Here, we describe and detail the use of sub-particle CryoEM averaging and present updated reconstructions of DARP14, a multi-subunit tetrahedrally symmetric protein complex. Originally described by Liu and Gonen et al. (2018), DARP14 was computationally designed as a scaffold capable of displaying small proteins for CryoEM. DARPins are small, ~17 kDa helical repeat proteins that feature variable residue loops capable of selective non-covalent binding to other proteins, akin to antibodies. Variants of DARP14 and similar scaffolds have since been generated and used to bind and image small proteins, such as GFP and KRAS.

In addition to focusing on the DARPin components, we also set out to extract as much high-resolution information as possible from the stable core cage component, this time by masking out the dynamic parts of the complex. To push for the highest resolution possible given the dataset, we created a mask that excluded the flexible DARPin components while keeping the core cage of DARP14 intact. Multiple rounds of 3D classifications and refinements using tetrahedral symmetry were made until no improvements to the map were observed. A final set of 277,091 particles were postprocessed using multiple rounds of Bayesian polishing and CTF refinement to obtain a final map of the core cage at 2.7 Å. At this resolution, we could model nearly every side chain of the complex. The map also shows possible sites of ions (mainly in the 3-fold trimeric interfaces) and water molecules (not modeled). At this point the resolution of the core cage is likely reaching the limits inherent to the sample and data collection parameters.

>[12x]KDSPIIEANGTLDELTSFIGEAKHYVDEEMKGILEEIQNDIYKIMGEIGSKGKIEGISEERIAWLLKLILRYMEMVNLKSFVLPGGTLESAKLDVCRTIARRALRKVLTVTREFGIGAEAAAYLLALSDLLFLLARVIEIE;>[12x]PHLVIEATANLRLETSPGELLEQANKALFASGQFGEADIKSRFVTLEAYRQGTAAVERAYLHACLSILDGRDIATRTLLGASLCAVLAEAVAGGGEEGVQVSVEVREMERLSYAKRVV> MAVPIAQKSEPHSLSSEALMRRAVSLVTDSTSTFLSQTTYALIEAITEYTKAVYTLTSLYRQ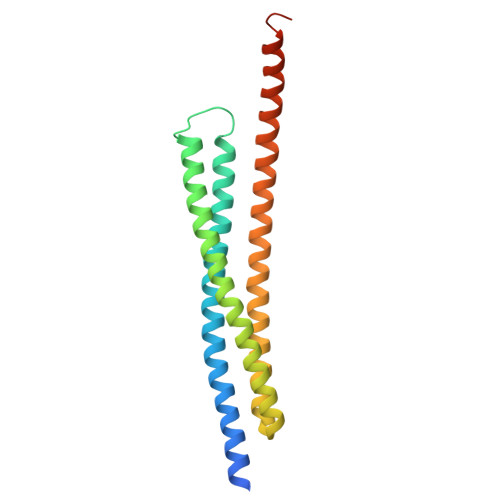YTSLLGKMNSEEEDEVWQVIIGARAEMTSKHQEYLKLETTWMTAVGLSEMAAEAAYQTGADQASITARNHIQLVKLQVEEVHQLSRKAETKLAEAQIEELRQKTQEEGEERAESEQEAYLREDHHHHHHHHH> TARIALASLFVVAAVLAQPWQTTTQRWVLGVSIAAVIVLLAWWKGMFLTTRIGRALAMVRRNRAEDTVETDAHRATVVLRVDPAAPAQLPVVVGYLDRYGITCDKVRITHRDAGGTRRSWISLTVDAVDNLAALQARSARIPLQDTTEVVGRRLADHLREQGWTVTVVEGVDTPLPVSGKETWRGVADDAGVVAAYRVKVDDRLDEVLAEIGHLPAEETWTALEFTGSPAEPLLTVCAAVRTSDRPAAKAPLAGLTPARGRHRPALAALNPLSTERLDGTAVPLPA;>VMPIVRVAVLAAGDDGGRLTEMALPSELPLREILPAVQRIVQPARENDGAADPAAAPNPVRLSLAPIGGAPFSLDATLDTVGVVDGDLLALQAVPSGPPAPRIVEDIADAAVIFSEARRRQWGPTHIARGAALALIGLILVGTGLSVAHRVITGDLLGQFIVSGIALATVIAALAVRNRSAVLATSLAVTALVPVAAAFALGVPGDFGAPNVLLAAAGVAAWSLISMAGSPDDRGIAVFTATAVTGVGVLLVAGAASLWVISSDVIGCALVLLGLIVTVQAAQLSAMWARFPLPVIPAPGDPTPAARPLSVLADLPRRVRVSQAHQTGVIAAGVLLGVAGSVALVSSANASPWAWYIVVAAAAGAALRARVWDSAACKAWLLGHSYLLAVALLVAFVIGDRYQAALWALAALAVLVLVWIVAALNPKIASPDTYSLPMRRMVGFLATGLDASLIPVMALLVGLFSLV[2x];> VTRHQVSGWRFVMRRIASGVALHDTRMLVDPLRTQSRAVLTGALILVTGLVGCFIFSLF;> MSRLIFEHQRRLTPPTTRKGTITIEPPPQLPMRTEEVDAERADYLRYLSVVRDNVRAHAAEQRAALEWSHPEPEVLATIPGTRRQWERDPRDRDFLVLRAGRHDVPLDAALKVKDTADEIDLEPVAHSALRGLLDVQRTVRDAPTGLDVAKLARITVIGEADEARAAIRAWIAQAVTWHDPTMLGVALAAPDLESGDWSWLKWLPHVDVPNEADGVGPARYLTTSTAELRERLAPALADRPLFPAE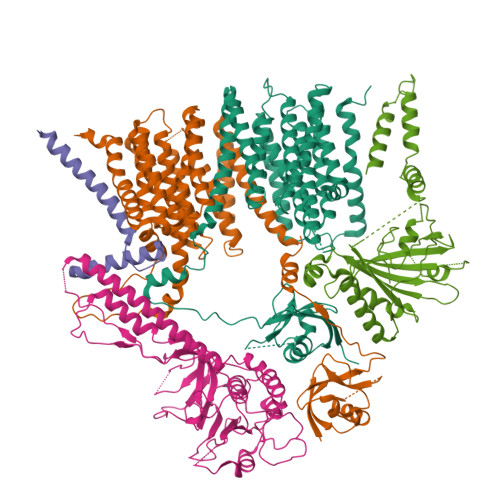SGAALKHLLVVLDDPDADPDDIARKPGLTGVTVIHRTTELPNREQYPDPERPILRVADGRIERWQVGGWQPCVDVADAMSAAEAAHIARRLSRWDSN> GSPGISGGGGGILLVANPVIPDVSVLISGPPIKDPEALLRYALPIDNKAIREVQKPLEDITDSLKIAGVKALDSVERNVRQASRTLQQGK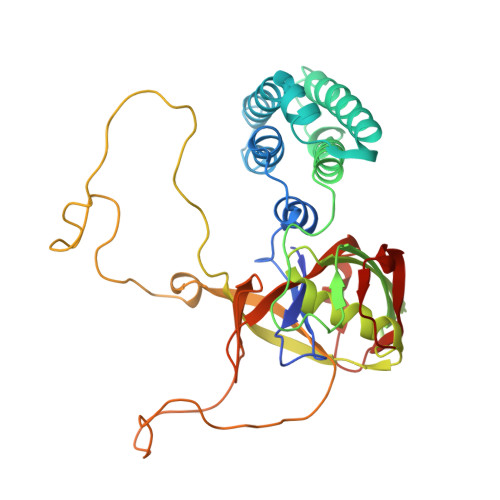SIIVAGFAESKKDHGNEMIEKLEAGMQDMLKIVEDRKRDAVAPKQKEILKYVGGIEEDMVDGFPYEVPEEYRNMPLLKGRASVDMKVKIKDNPNIEDCVFRIVLDGYNAPVTAGNFVDLVERHFYDGMEIQRSDGFVVQTGDPEGPAEGFIDPSTEKTRTVPLEIMVTGEKTPFYGSTLEELGLYKAQVVIPFNAFGTMAMAREEFENDSGSSQVFWLLKESELTPSNSNILDGRYAVFGYVTDNEDFLADLKVGDVIESIQVVSGLENLANPSYKIAG> MALDRPDRSGAVRVSAPARLSFTAISLDGSSLRRNGIAAMAVDRPGLTAEVREAADGIVAVTGTAEETARELAAALEALRKLWDGPAARVDVLEALPQHSGFGSKTSTLLAVGHAYGRLCGVEPDLRELARTLGRGRTSGASTGLSAYGGFLVDGGHVNPPDFAEAPQKYLRPSRFAQQVAPPKPVVRLDFPDWPVLVLLTHGRHLGGQEELEWFHSVAPIPAEESWRTSHLVFMGLAPAVLEQDFDAFCAAVNEITFTGHFKQAQIAFQGDAVADVLEAGRAAPSVDAIALSVTGPACFAFTKRPEDAERWAWELKNRGLIRDFWFTRANNQGLATTVVS

In the specific case of formycin, the enzyme ForT catalyses C-C bond formation between 4-amino-1H-pyrazole-3,5-dicarboxylate (APDA) and PRPP, in a reaction that is driven by the elimination of CO2 and inorganic pyrophosphate (PPi). ForT catalyses C-C bond formation in formycin A biosynthesis, and we have previously determined its structure complexed to PRPP. This structure establishes that ForT is a member of the GHMP kinase superfamily. ITC measurements show that APDA binds to ForT only in the presence of PRPP, suggesting that the reaction likely follows an ordered bi-bi kinetic mechanism in which PRPP binds first and creates the binding site for APDA. Glu211 is essential for catalysis, and we suggest it acts as a general base to make APDA sufficiently nucleophilic.

By contrast, the L24A variant exhibits only a small reduction in kcat but a 20-fold reduction in affinity for APDA on the basis of both the KM and KD values. We were also able to observe structural changes that take place as a result of catalysis by solving the X-ray crystal structure of the L24A/CAPR/PPi product complex to 1.75 Å resolution in space group P41212. The protein structure in the product complex is almost identical to that seen in the binary complex (RMSD of 0.41 Å over 319 overlapping Cα atoms). The loop at Ser174 is disordered here similar to the binary complex and in contrast with the T138V/APDA/MgPRPP ternary complex. The location of free pyrophosphate (consequently its interaction with the protein) is identical to the pyrophosphate portion of PRPP in the ternary complex. The Mg2+-binding site has been eliminated, however, because the CAPR ribose ring occupies a position intermediate between those seen in the ternary and binary complexes. As a result, the 2′-OH and 3′-OH groups hydrogen bond to the Thr138 side chain and a water molecule, respectively. The single carboxylate group of CAPR hydrogen bonds to the side chains of Ser21 and Gln266, in a similar manner to that seen for that cognate group in the T138V/APDA/MgPRPP ternary complex although the carboxylate atoms are shifted between 0.6 and 1.2 Å. The heterocyclic ring of CAPR is ‘flipped’ relative to the APDA and the extracyclic amine is within hydrogen bonding distance of a water molecule, but this water does not bridge to E211. The simplest explanation is this orientation is a feature of the L24A variant used to obtain the structure.> MALAKRIDAALIMKDGRVVKGSNFENLRDSGDPVELGKFYSEIGIDELS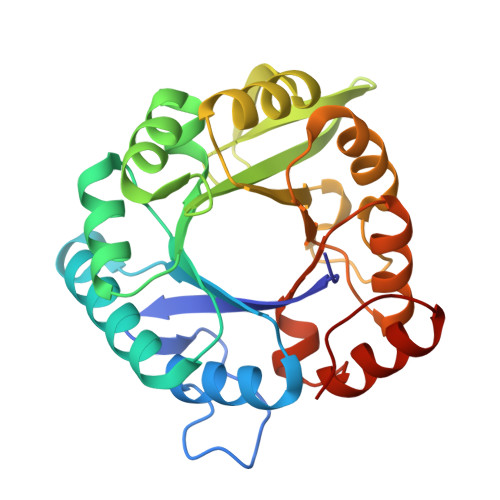FWDITASVEKRKTMLELVEKVAEQIDIPFTVGGGIHDFETASELILRGADKVEINTAAVENPSLITQIAQTFGSQAVVVYIAAKRVDGEFMVFTYSGKKNTGILLRDWVVEVEKRGAGEIVLGSIDRLGTKSGYDTEMIRFVRPLTTLPIIAHRGAGKMEHFLEAFLAGADAAKADSVFHFREIDVRELKEYLKKHGVNVRLE> MGSDKIHHHHHHENLYFQGMTKAIQSSVQVGELATGQALTVPIYSFMGSENSAPSVYIQANVHGAEVQGNAVIYQLMTLLEGYQVLGDITLAPLANPLGINQKSGEFTLGRFDPITGVNWNREYFDHNVDIQNWYAEHQHLTNSELFCAYRSMLVETCQARLTHSFGISTGHRLAVNLQAMAHQADIVLDLHTGPKSCKHLYCPEYDIDAARFFSIPYTLIIPNSFGGAMDEATFCPWWQL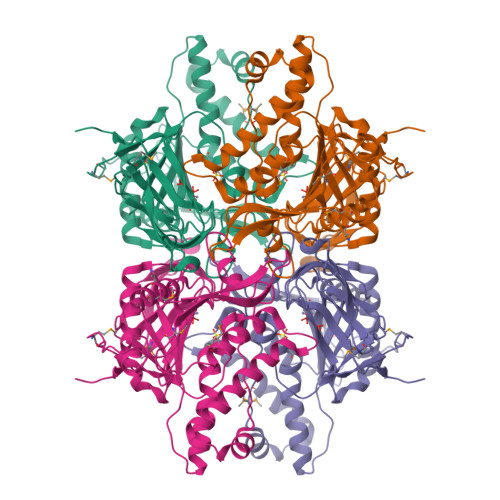TEYATSQGREFSVPVSAFTLELASQERIDLADALEDAKGILAYLSHRGVIAEKVNPASMERFGCYLKDYKKFHAPKAGLIEYCASVGEPLTAGKPLVNILRIDLYGSEQAYQAISLPMDCVPILHFASASVLQGTELYKVMTNVFPLQPS In this context, the plant caseinolytic protease (Clp) complex plays an important role in degradation of accumulated and misfolded proteins in chloroplasts wherein the chaperones aid in ATP-dependent unfolding of protein substrates to be degraded by the associated protease machinery. The structured, mature forms of AtClpC1/C2/D consist of three distinct domains such as a short N-terminal domain (NTD) and two ATPase domains, a feature very similar to bacterial ClpC proteins. The N-terminal domain of ClpC1 is known to perform the regulatory function of substrate recognition, either directly or indirectly through the adaptor proteins ClpS1/ClpF for which it becomes a binding platform161718, whereas no adaptor proteins have so far been reported for ClpD. Here we report and analyse the crystal structures of AtClpC1 residues 94 to 238 and AtClpD residues 79 to 233 (hereafter mentioned as AtClpC1 NTD and AtClpD NTD respectively) that correspond to the ClpC NTD of eubacteria.

The 1.6 Å structure of AtClpD N-terminal domain (residues 79–233) revealed a α-helical structure, having 61% helical content. The domain is made up of seven helices: α1 (E85-L101), α2 (T106-E118), α3 (I132-D144), α4 (I170-M186), α5 (P191-V203), α6 (S207-L215) and α7 (M219-K231). The crystal structure included two molecules in an asymmetric unit. The crystal structure additionally shows the 26-residue long middle loop to take a different conformation compared to the 14-residue long loop of AtClpC1 NTD. Also, unlike in AtClpC1, the two halves of AtClpD NTD do not form the typical four-helix motif repeats. In AtClpD, residues 122–128, which makes the short stretch corresponding to α3 of AtClpC1 NTD forms a loop instead of helix. The fact that there are helix breaker residues such as a Pro and two Gly within this stretch supports the experimental evidence for the presence of loop instead of a helix. The presence of longer middle loop and the absence of a helix in the stretch corresponding to α3 of AtClpC1 NTD make AtClpD NTD very different from any known Clp chaperone NTD structures and perhaps might attribute its functional significance of having to recognize specific substrates during stress conditions, without the involvement of any adaptor proteins. When the structure of AtClpD NTD is aligned with AtClpC1 NTD, we realize that the long middle loop comes directly over the region which may otherwise contribute to ClpS1 interaction. Therefore, AtClpD not binding to AtClpS1 or AtClpF could at least partly be due to the presence of the long middle loop in AtClpD NTD which would sterically prevent any such interaction.

>PLGSMVFERFTERAIRAIIFSQKEAKSLGKDMVYTQHLLLGLIAEDRDPQGFLGSGITIDKAREAVWSIWDEANSDSKQEEASSTSYSKSTDMPFSISTKRVFEAAVEYSRTMDCQYIAPEHIAVGLFTVDDGSAGRVLKRLGANMNLLTAAALTRLKGE[2x]~{N}-(4,4-dimethyl-2-propyl-3,1-benzoxazin-6-yl)-2-[3-methoxy-5-(7-methoxyquinolin-4-yl)oxy-pyridin-2-yl]ethanamide 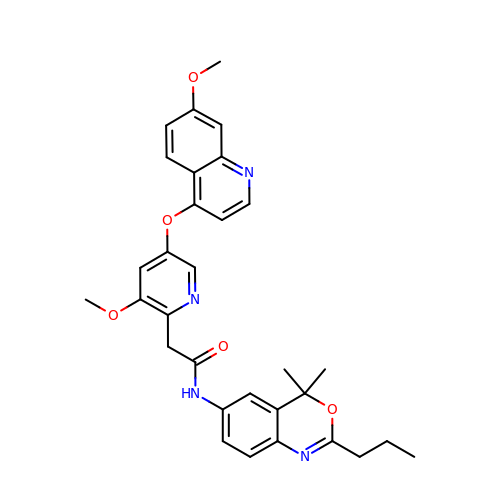| C31 H32 N4 O5 | WBUHTZNBWYBTSN-UHFFFAOYSA-N4-butyl-5-propyl-1,3-selenazol-2-amine | C10 H18 N2 Se | 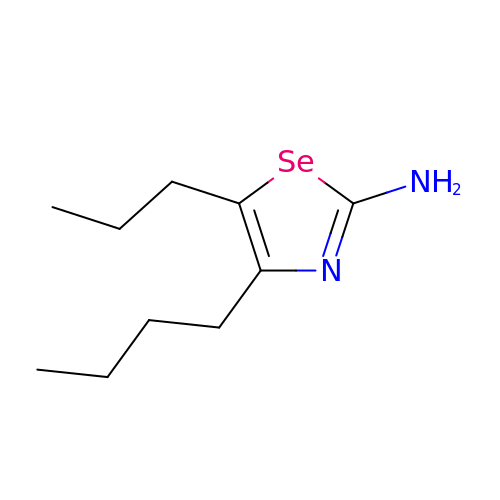DOUUMUUUWUAPPC-UHFFFAOYSA-N ethyl 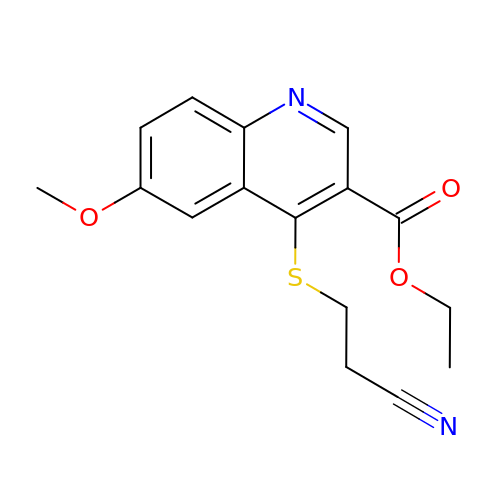4-(2-cyanoethylsulfanyl)-6-methoxy-quinoline-3-carboxylate | C16 H16 N2 O3 S | TZDUQSHGGUOAJU-UHFFFAOYSA-N> MNYTETVAYIHSFPRLAKTGDHRRILTLLHALGNPQQQGRYIHVTGTNGKGSAANAIAHVLEASGLTVGLYTSPFIMRFNERIMIDHEPIPDAALVNAVAFVRAALERLQQQQADFNVTEFEFITALGYWYFRQRQVDVAVIEVGIGGDTDSTNVITPVVSVLTEVALDHQKLLGHTITAIAKHKAGIIKRGIPVVTGNLVPDAAAVVAAKVATTGSQWLRFDRDFSVPKAKLHGWGQRFTYEDQDGRISDLEVPLVGDYQQRNMAIAIQTAKVYAKQTEWPLTPQNIRQGLAASHWPARLEKISDTP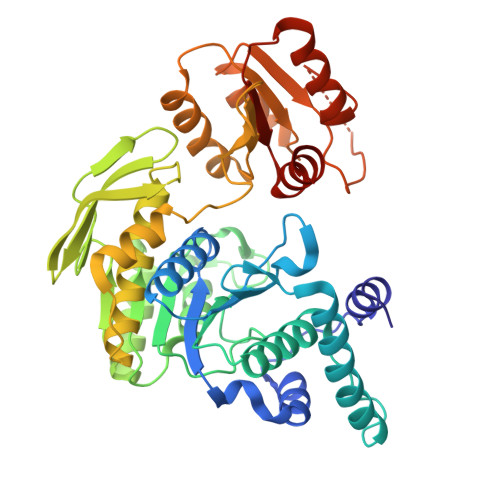LIVIDGAHNPDGINGLITALKQLFSQPITVIAGILADKDYAAMADRLTAAFSTVYLVPVPGTPRALPEAGYEALHEGRLKDSWQEALAASLNDVPDQPIVITGSLYLASAVRQTLLGGKS> MNQRLMTGDAMQANFGFVTSQTAYVEAGVYRMRYPEIRYPGLIPVDYSAPEWIKTVDYYSMDGVGKAE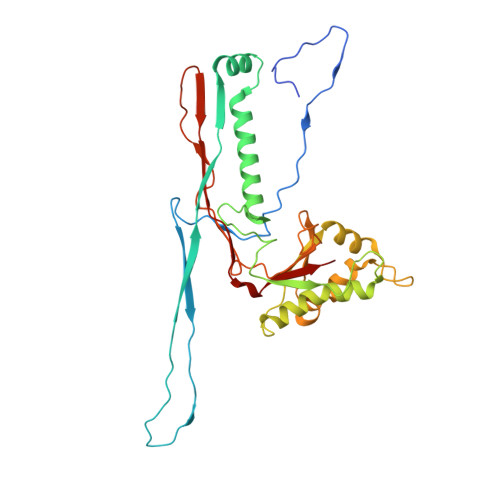WIADRASDIPVVGLAMEKATTTVHLAGIGYDYGLEEVNQAIMLGMNLPGEKANLARLVYERMVDRVAFTGDAEKDFKGLFNNGAVTAVSATTGNWASATADQILADFNLGITGLWSATNEMVYADTVLLPSAKHQIIASKRLGNEATETVLQFLQRANVYTAETGRPLTIRGMRGLNTAGAGGVSRSVFYRNSPEVLKMHIPMRHRFLPVQVVGLTYKVPGIFRLGGLDIRLPKEVRYVDGY>[2x]MPLPKTHELHIFGSFNGVKFDMVGEGTGNPNEGSEELKLKSTNGPLKFSPYILVPHLGYGFNQYLPFPDGMSPFQAAMQDESGYQVHRTLQYEDGAFVTANLRYTYEGS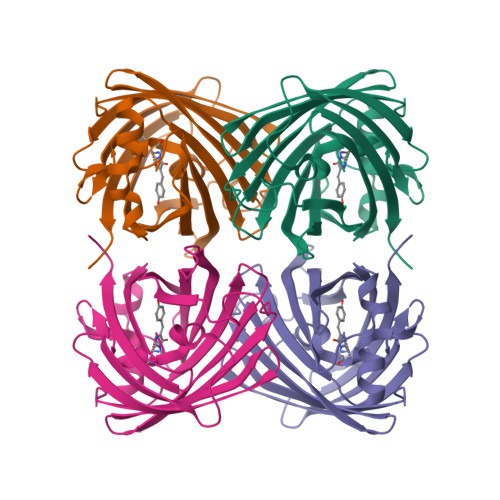HIKGEFQVIGTGFPPDGPVMTNKLTALDWSVVKFVYPNDKTILSTFDKTYTTTDGKRYQCTFRENNTFAKPMAADILQKQPMFIFHKTELQHSNNAELTFKEKQTAFSDMKSGGSHHHHHH> GIGAVLKVLTTGLPA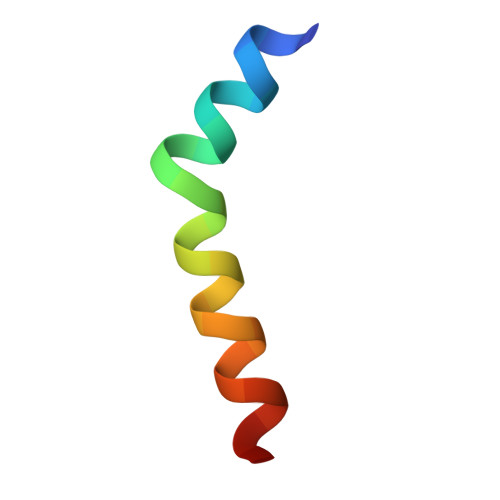LISWIKRKRQQX The UbiD superfamily is composed of a wide variety of (de)carboxylases acting on aromatic, hetero-aromatic, and unsaturated aliphatic acids. Prenylated FMN consists of an FMN molecule modified by the addition of a fourth non-aromatic ring joined via N5–C1′ and C6–C3′ linkages between the flavin and prenyl moieties. Following binding of prFMNreduced and formation of holo-UbiD, the cofactor undergoes oxidation to form the catalytically relevant oxidized prFMN species. In the UbiD enzyme family, Arg173, Glu277, and Glu282 (A. niger Fdc1 numbering) form a conserved ionic network.

Crystallization of wildtype, E285D, and R175A S. cerevisiae Fdc1 variants confirms cofactor incorporation. E285D exhibits minimal disruption to the active-site architecture, with hydrogen-bonding distances remaining very similar to those of wildtype and prFMN lacking modification on the C1′. For E285D kcatapp has been measured as 0.28 ± 0.01 s−1, and Kmapp has been measured as 20.4 ± 3.6 μm. Movement of residue 282 during the catalytic cycle of Fdc1 could therefore facilitate the shuttling of protons between solvent and the active site. Both the E282Q (A. niger) and E285Q (S. cerevisiae) variants are inactive, whereas E282D and E285D variants retain a considerable level of decarboxylase activity. Furthermore, the pH dependence of the reaction for both Glu → Asp variants is similar to that observed for the WT. This suggests the pKa of key groups involved in catalysis is unperturbed by the Glu → Asp substitution, with the lower kcat values observed for E282D and/or E285D possibly resulting from increased proton transfer distances, as the carboxylate group is slightly shifted in crystal structures of these variants.

>[4x]MRKLNPALEFRDFIQVLKDEDDLIEITEEIDPNLEVGAIMRKAYESHLPAPLFKNLKGASKDLFSILGCPAGLRSKEKGDHGRIAHHLGLDPKTTIKEIIDYLLECKEKEPLPPITVPVSSAPCKTHILSEEKIHLQSLPTPYLHVSDGGKYLQTYGMWILQTPDKKWTNWSIARGMVVDDKHITGLVIKPQHIRQIADSWAAIGKANEIPFALCFGVPPAAILVSSMPIPEGVSESDYVGAILGESVPVVKCETNDLMVPATSEMVFEGTLSLTDTHLEGPFGDMHGYVFKSQGHPCPLYTVKAMSYRDNAILPVSNPGLCTDETHTLIGSLVATEAKELAIESGLPILDAFMPYEAQALWLILKVDLKGLQALKTTPEEFCKKVGDIYFRTKVGFIVHEIILVADDIDIFNFKEVIWAYVTRHTPVADQMAFDDVTSFPLAPFVSQSSRSKTMKGGKCVTNCIFRQQYERSFDYITCNFEKGYPKGLVDKVNENWKRYGYKHHHHHH> MGSLTEDGLSYKEKFVVRSYEVGSNKTATVETIANLLQEVGCNHAQSVGFSTDGFATTTTMRKLHLIWVTARMHIEIYKYPAWGDVVEIETWCQSEGRIGTRRDWILKDSVTGEVTGRATSKWVMMNQDTRRLQKVSDDVRDEYLVFCPQEPRLAFPEENNRSLKKIPKLEDPAQYSMIGLKPRRADLDMNQHVNNVTYIGWV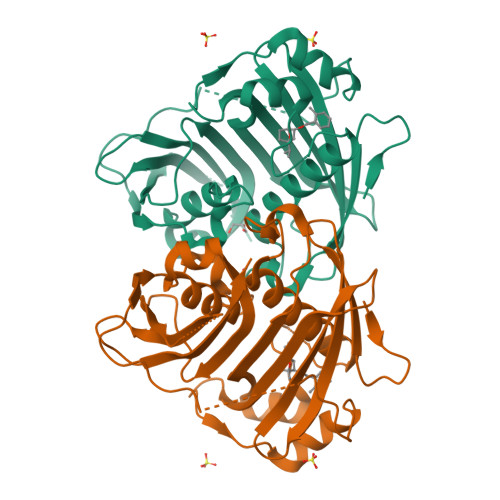LESIPQEIVDTHELQVITLDYRRECQQDDVVDSLTTTTSEIGGTNGSATSGTQGHNDSQFLHLLRLSGDGQEINRGTTLWRKKPSSHHHHHH>NLGAAVAILGGPGTV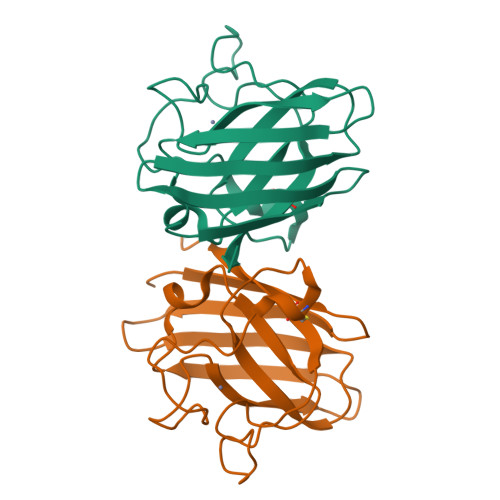QGVVRFLQLTPERCLIEGTIDGLEPGLHGLHVHQYGDLTNNCNSCGNHFNPDGASHGGPQDSDRHRGDLGNVRADADGRAIFRMEDEQLKVWDVIGRSLIIDEGEDDLGRGGHPLSKITGNSGERLACGIIARSAGL[2x]> GSMTGPGALS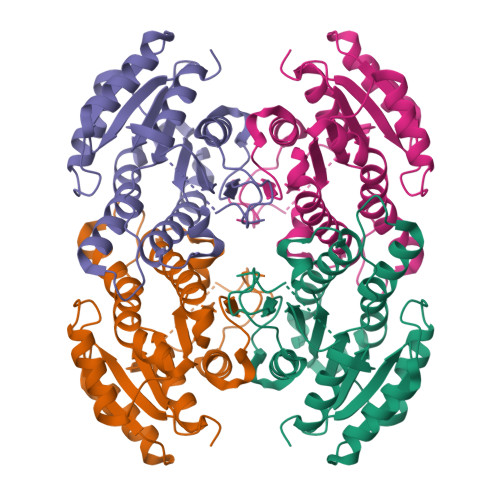GKVALVTGGSRGLGRAMALRLARDGAAVAIVYVSDDSSAKETQGEIERLGGTARSYRCDVSDAEQVTRCVKAVTADLGPVDILVNNAGIIRDGLAASIKDEDYDAVMNTNLKGAFLFIKACYFGFIRKRSGSIINISSVSGVFGSAGQANYASAKAGLIGLTKSIAKELAERNVRCNAVAPGLIATDMTQDLVDDSKRLDPVPMRRFGRPDEVAGLVAFLAGDESSYITGQVVCVDGGMAM>[4x]MGSSHHHHHHSSGENLYFQGVPTVQRGIIKMVLSGCAIIVRGQPRGGPPPERQINLSNIRAGNLARRAAKDTPDEPWAFPAREFLRKKLIGKEVCFTIENKTPQGREYGMIYLGKDTNGENIAESLVAEGLATRREGMRANNPEQNRLSECEEQAKAAKKGMWSEGN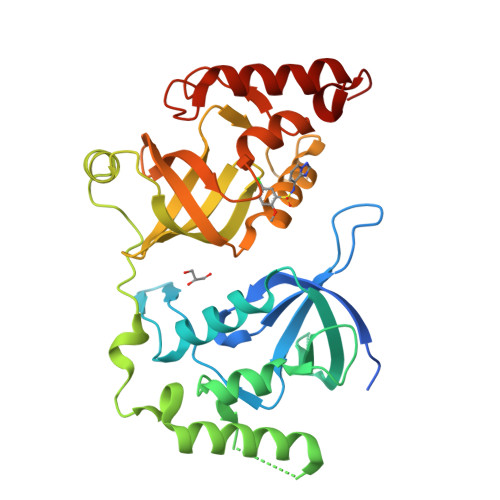GSHTIRDLKYTIENPRHFVDSHHQKPVNAIIEHVRDGSVVRALLLPDYYLVTVMLSGIKCPTFRRETPEPFAAEAKFFTESRLLQRDVQIILESCHNQNILGTILHPNGNITELLLKEGFARCVDWSIAVYTRGAEKLRAAERFAKERRLRIWRDYV>GIPRRITKETQNLANEPPPGIMAVPVPENYRHFNILINGPDGTPYEGGTYKLELFLPEQYPMEPPKVRFLTKIYHPNIDKLGRICLDILKDKWSPALQIRTVLLSIQALLSSPEPDDPLDSKVAEHFKQDKNDAEHVARQWNKIYANNNVL[2x];> MHHHHHHSSGRENLYFQGMSEVIVPRSFRLLDELERGQKGNVSEGVSFGLESADDITLSNWSCTIFGQPGTVFENRIYSLTIFCDDNYPDSPPTVKFDTKIE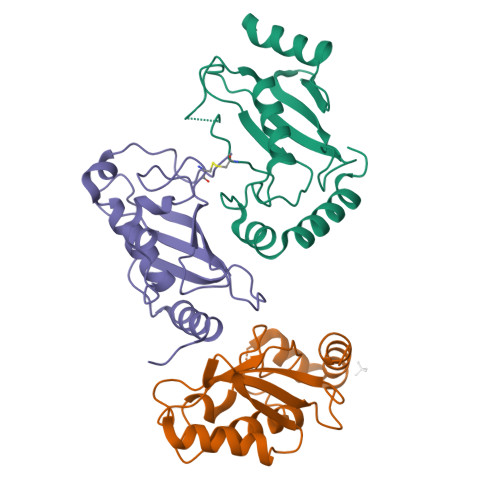MSCVDNCGRVIKNNLHILKNWNRNYTIETILISLRQEMLSSANKRLPQPNEGEVYS>MADADLDKQVNTAGAWPIATGGYYSQHNSPLAQINKSNVKNVKAAWSFSTGVLNGHEGAPLVIGDMMYVHSAFPNNTYALNLNDPGKIVWQHKPKQDASTKAVMCCDVVDRGLAYGAGQIVKKQANGHLLALDAKTGKINWEVEVCDPKVGSTLTQAPFVAKDTVLMGCSGAELGVRGAVNAFDLKTGELKWRAFATGSDDSVRLAKDFNSANPHYGQFGLGTKTWEGDAWKIGGGTNWGWYAYDPKLNLFYYGSGNPAPWNETMRPGDNKWTMTIWGRDLDTGMAKWGYQKTPHDEWDFAGVNQMVLTDQPVNGKMTPLLSHIDRNGILYTLNRENGNLIVAEKVDPAVNVFKKVDLKTGTPVRDPEFATRMDHKGTNICPSAMGFHNQGVDSYDPESRTLYAGLNHICMDWEPFMLPYRAGQFFVGATLAMYPGPNGPTKKEMGQIRAFDLTTGKAKWTKWEKFAAWGGTLYTKGGLVWYATLDGYLKALDNKDGKELWNFKMPSGGIGSPMTYSFKGKQYIGSMYGVGGWPGVGLVFDLTDPSAGLGAVGAFRELQNHTQMGGGLMVFSL[2x];>YDGQNCKEPGNCWENKPGYPEKIAGSKYDPKHDPVELNKQEESIKAMDARNAKRI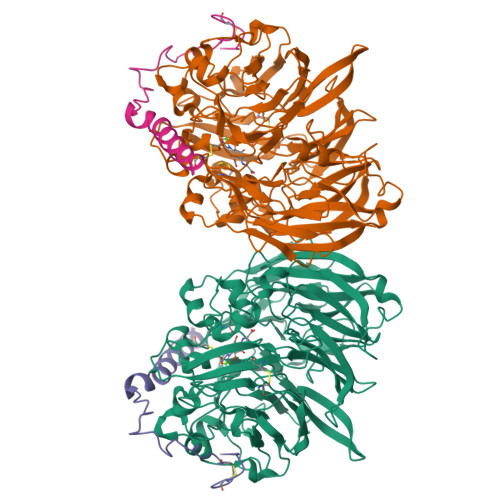ANAKSSGNFVFDVK[2x]> TQKPSLYRVLILNDDYTPMEFVVYVLERFFNKSREDATRIMLHVHQNGVGVCGVYTYEVAETKVAQVIDSARRHQHPLQC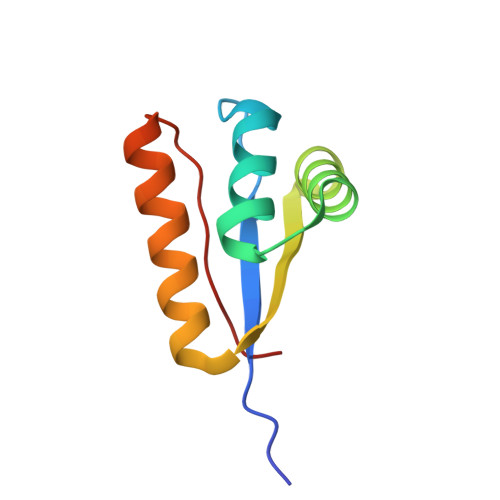TMEKD> MGHHHHHHGRADGGFRPSRVVVVAKTTRYEFEQQRYRYAELSEEDLKQLLALKGSSYSGLLERHHIHTKNVEHIIDSLRNEGIEVRLVKRREYDEETVRWADAVIAAGGDGTMLLAASKVLDRLKPVIGVNTDPERSEGHLCLPVRYTHSFPEALQKFYRGEFRWLWRQRIRLYLEGTGINPVPVDLHEQQLSLNQHNRALNIERAHDERSEASGPQLLPVRALNEVFIGESLSSRASYYEISVDDGPWEKQKSSGLNLCTGTGSKAWSFNINRVATQAVEDVLNIAKR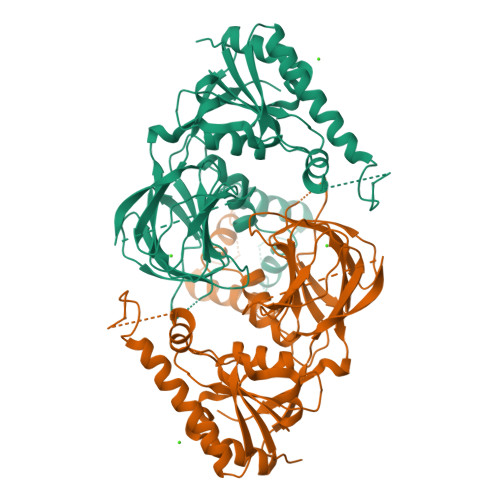QGNLSLPLNRELVEKVTNEYNESLLYSPEEPKILFSIREPIANRVFSSSRQRCFSSKVCVRSRCWDACMVVDGGTSFEFNDGAIASMMINKEDELRTVLLEQ>[6x]GSMTREASPGASPEHAFRFHHIGVQTSDLENSLGWYREFFGCEQNWSLEKFSDLTRSRLPGITR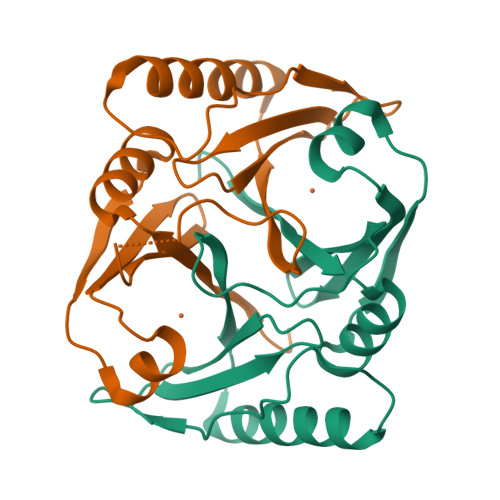LVELAAGDLRIHVFERAADATPAPVAEVPQFQHLCLATRSPEEMTEWRDRWLELYESGRYTFVRDEGPTDIVVDEDGVLSLYVLDVNGLEYEFTYLPEGVE>MNKKLIIPFALAPLAAPALQAQSQQSDGRMDTRPNIILFMVDDMGWQDTSLPFWTQKTHYNEVYETPNMERLAKQGVMFTQAYASSICSPTRCSLITGTNAARHRVTNWTYPKGQQTDRPSDVFNVADWNVNGVCQVPNIDHTFQATSLAEILKDNGYHTIHCGKAHFGAVNTPGESPYHMGFEVNIAGHAGGGLASYLGENNYGNRTDGKPNPWFAVPGLDKYWGTDTFVSEALTLEAIKALNHAKEYNQPFFLYMAHYAIHVPIDKDKRFYQKYIDKGLTPKEAAYAALIEGMDKSLGDLMDWLDKNGEADNTIVIFMSDNGGLSSEPGWRDGKLHTQNSPLNSGKGSAYEGGVREPMIVRWPGVVKPDTKCDKYLIIEDFYPSILEMAQVKHYKTVQPIDGISFIPLLKQTGDPSKGRSLYWNFPNHWGNDGPGIGPT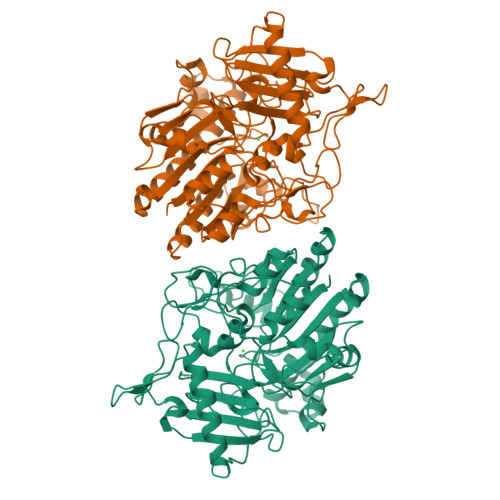CTVRKGDWKLIYYYENGKKELFNIPQDIGEKNNLAAQHPDIVKHLSKDLGNYLRKVGGQRPSFKATGKPCPWPDEI[2x]>SANEVIKCKAAVAWEAGKPLSIEEIEVAPPKAHEVRIKIIATAVCHTDAYTLSGADPEGCFPVILGHEGAGIVESVGEGVTKLKAGDTVIPLYIPQCGECKFCLNPKTNLCQKIRVTQGKGLMPDGTSRFTCKGKTILHYMGTSTFSEYTVVADISVAKIDPLAPLDKVCLLGCGISTGYGAAVNTAKLEPGSVCAVFGLGGVGLAVIMGCKVAGASRIIGVDINKDKFARAKEFGATECINPQDFSKPIQEVLIEMTDGGVDYSFECIGNVKVMRAALEACHKGWGVSVVVGVAASGEEIATRPFQLVTGRTWKGTAFGGWKSVESVPKLVSEYMSKKIKVDEFVTHNLSFDEINKAFELMHSGKSI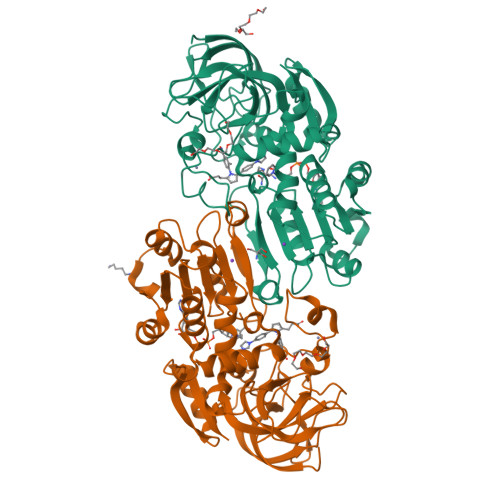RTVVKI[2x]> GPRGCPTHCHCEPDGRMLLRVDCSDLGLSELPSNLSVFTSYLDLSMNNISQLLPNPLPSLRFLEELRLAGNALTYIPKGAFTGLYSLKVLMLQNNQLRHVPTEALQNLRSLQSLRLDANHISYVPPSCFSGLHSLRHLWLDDNALTEIPVQAFRSLSALQ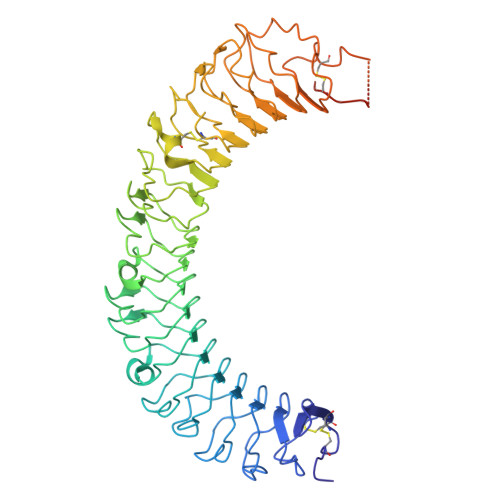AMTLALNKIHHIPDYAFGNLSSLVVLHLHNNRIHSLGKKCFDGLHSLETLDLNYNNLDEFPTAIRTLSNLKELGFHSNNIRSIPEKAFVGNPSLITIHFYDNPIQFVGRSAFQHLPELRTLTLNGASQITEFPDLTGTANLESLTLTGAQISSLPQTVCNQLPNLQVLDLSYNLLEDLPSFSVCQKLQKIDLRHNEIYEIKVDTFQQLLSLRSLNLAWNKIAIIHPNAFSTLPSLIKLDLSSNLLSSFPITGLHGLTHLKLTGNHALQSLISSENFPELKVIEMPYAYQCCAFGVCENAYKISNQWNKGDNSSMDDLHKKDAGMFQAQDERDLEDFLLDFEEDLKALHSVQCSPSPGPFKPCEHLLDGAAA Full-length MLL5 is a 205 kDa protein (1858 residues), although a smaller isoform (around 75 kDa) including a single Plant HomeoDomain (PHD) and a Su(var)3-9, Enhancer of zeste, Trithorax (SET) domain has been described. Even if a hallmark of SET domain-containing proteins is the histone methyltransferase (HMT) activity, it remains controversial whether the human and mouse MLL5 SET domains possess a catalytic HMT activity. To better understand the molecular mechanism of human MLL5 function, we solved the crystal structure of its SET domain at 2.1 Å resolution. Accordingly, biochemical and biophysical experiments showed that the SET domain of MLL5 is devoid of any binding activity towards histone peptides or the cofactor S-Adenosyl Methionine (SAM) in vitro and does not exhibit HMT activity on full-length histones.

The SET domain alone (residues 323 to 458) crystallized in the space group P3121, and diffracted up to 2.1 Å resolution. To allow crystallization, we mutated an exposed and non-conserved cysteine (Cys 453) into alanine since this residue caused heterogeneity of the protein due to dimerization by formation of an intermolecular disulfide bridge. The final crystal structure of the SET domain of MLL5 in its free form was refined at 2.1 Å resolution with an R-factor equal to 20.9% and R-free equal to 24.2% with good stereochemistry. The asymmetric unit contained two unliganded MLL5 molecules which superposed with a root mean square deviation (RMSD) of 0.64 Å (110 Cα atoms). The overall tertiary structure of the MLL5 SET domain is similar to that of previously determined SET domain structures. A unique structural feature of the SET domain of MLL5 is a very short helix α1 (two turns, from Arg 365 to Asn 371) where other SET domains usually display a four-turn α-helix (e.g. DIM-5 and MLL3). Accordingly, the shortening of this helix results in the formation of a long loop (from Gly 372 to Phe 381) that is very uncommon in SET domains. This large loop between α1 and β5 occupies a groove which, in other SET domains, serves as a substrate docking site. However, contrary to MLL5, the elongated loops of these methyltransferases sit outside of the domain. It is noteworthy that this MLL5-specific loop conformation is observed in both molecules of the asymmetric unit and does not rely on crystallographic constraints. Indeed, the β1-β2 loop is disordered in the crystal structure, suggesting a high flexibility of this region.

>GPTNNLLFKPPVESHIQKNKKILKSAKDLPPDALIIEYRGKFMLREQFEANGYFFKRPYPFVLFYSKFHGLEMCVDARTFGNEARFIRRSCTPNAEVRHEIQDGTIHLYIYSIHSIPKGTEITIAFDFDYGNAKYKVD[2x]> MTLELQLKHYITNLFNLPKDEKWECESIEEIADDILPDQYVRLGALSNK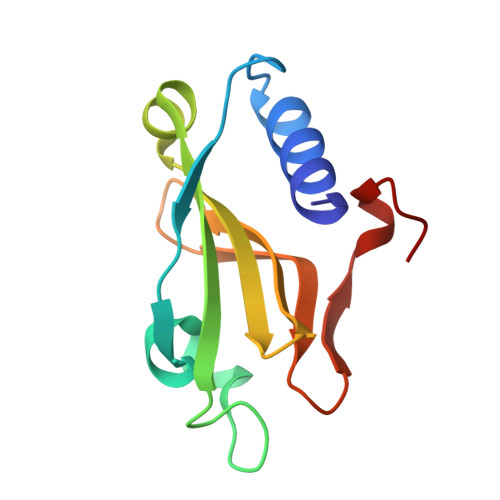ILQTYTYYSDTLHESNIYPFILYYQKQLIAIGYIDENHDMDFLYLHNTIMPLLDQRYLLTGGQ>[2x]MTAVQLIVGLGNPGPEYDQTRH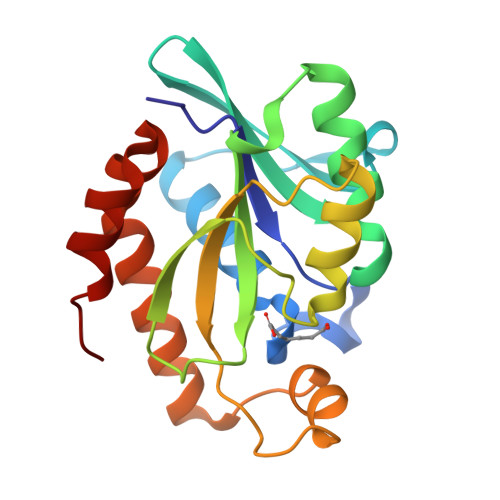NAGALFVERLAHAQGVSLVADRKYFGLVGKFSHQGKDVRLLIPTTYMNRSGQSVAALAGFFRIAPDAILVAHDELDMPPGVAKLKTGGGHGGHNGLRDIIAQLGNQNSFHRLRLGIGHPGHSSLVSGYVLGRAPRSEQELLDTSIDFALGVLPEMLAGDWTRAMQKLHSQKA> MKQLKWRTVNPEETKAIAKLTAAFAKPGDVLTLEGDLGAGKTTFTKGFAEGLGITRIVNSPTFTIIKEYNDGVLPLYHMDVYRMEDESED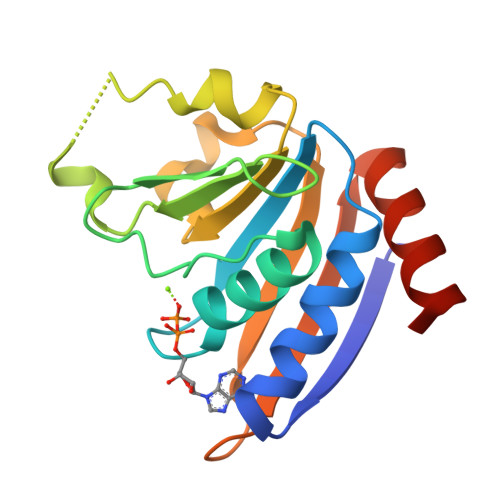LGLDEYFHGQGVCLVEWAHLIEEQLPQERLQIVIKRAGDDEREITFTAVGNRYEMLCEELSRHDNISN> SIIQVTFIAGRTELQKERLIAALTDAAVDTVGIERAEVRVILKDIPNTDYGIAGQT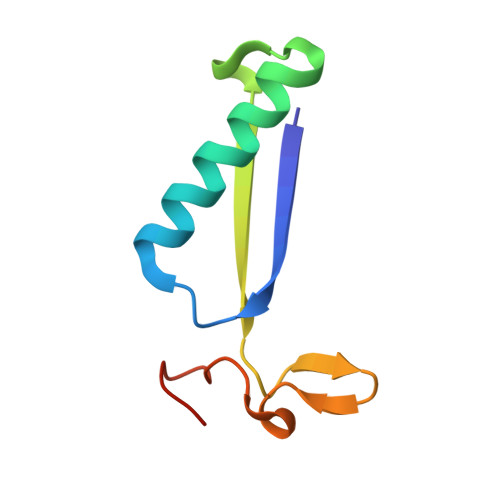ARSLGRGVDRHGRAPGGS Prostate-specific membrane antigen (PSMA) is a type II transmembrane glycoprotein specifically overexpressed in most PCa with limited expression in normal tissue. It is regarded as a high-value biomarker for PCa and has received worldwide attention for PCa diagnosis and treatment. Fluorescent molecular rotors (FMRs) are a family of fluorophores sensitive to local microenvironment (e.g., polarity and viscosity). In this study, we aimed at the design of activatable probes by linking a benzonitrile fluorescent rotor to the Lys-Urea-Glu scaffold, a well-established PSMA-targeting moiety used clinically for PCa imaging and radiotherapy.

To provide mechanistic rationale for the fluorescent enhancement of Glu-490 upon rhPSMA binding, we solved the crystal structure of the rhPSMA/Glu-490 complex and refined it to the 1.73 Å resolution limit. The active-site-bound Glu-490 was fitted into well-defined interpretable Fo-Fc electron density peaks in the final stages of the refinement. Positioning of the Lys-Urea-Glu motif is virtually indistinguishable from rhPSMA/urea ligand complexes reported previously. The FMR moiety consists of a distal N-substituted tetrahydroquinoline donor group, a thiophene ring spacer and a nitrile acceptor group. In our structure, the three subgroups adopt a near-planar configuration that is sustained via intermolecular interactions with PSMA residues. That spatial arrangement prevents the intramolecular twisting motion of the subgroups relative to each other and such rigidity is critical for efficient fluorescence emission upon FMR photoexcitation. The nitrile group is inserted into a deep pocket delineated the main chains of G206–F209 and the Y700 side chain. Furthermore, the FMR ring system is propped against the PSMA surface delineated by residues N698–G702 of the “glutarate sensor”. Here, the most conspicuous are CH–π interactions between the thiophene ring and the Y700 methylene group (4.0 Å) and the tetrahydroquinoline moiety and the A701 side chain methyl group (3.8 Å and 4.1 Å).

> KSSNEATNITPKHNMKAFLDELKAENIKKFLYNFTQIPHLAGTEQNFQLAKQIQSQWKEFGLDSVELAHYDVLLSYPNKTHPNYISIINEDGNEIFNTSLFEPPPPGYENVSDIVPPFSAFSPQGMPEGDLVYVNYARTEDFFKLERDMKINCSGKIVIARYGKVFRGNKVKNAQLAGAKGVILYSDPADYFAPGVKSYPDGWNLPGGGVQRGNILNLNGAGDPLTPGYPANEYAYRRGIAEAVGLPSIPVHPIGYYDAQKLLEKMGGSAPPDSSWRGSLKVPYNVGPGFTGNFSTQKVKMHIHSTNEVTRIYNVIGTLRGAVEPDRYVILGGHRDSWVFGGIDPQSGAAVVHEIVRSFGTLKKEGWRPRRTILFASWDAEEFGLLGSTEWAEENSRLLQERGVAYINADSSIEGNYTLRVDCTPLMYSLVHNLTKELKSPDEGFEGKSLYESWTKKSPSPEFSGMPRISKLGSGNDFEVFFQRLGIASGRARYTKNWETNKFSGYPLYHSVYETYELVEKFYDPMFKYHLTVAQVRGGMVFELANSIVLPFDCRDYAVVLRKYADKIYSISMKHPQEMKTYSVSFDSLFSAVKNFTEIASKFSERLQDFDKSNPIVLRMMNDQLMFLERAFIDPLGLPDRPFYRHVIYAPSSHNKYAGESFPGIYDALFDIESKVDPSKAWGEVKRQIYVAAFTVQAAAETLSEVA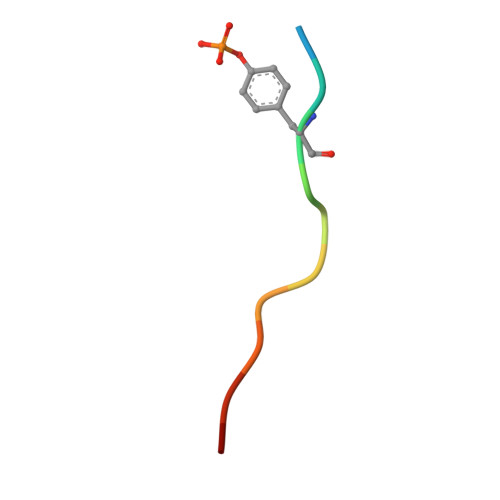> ANSYENVLIAKX> QSACTLQSETHPPLTWQKCSSGGTCTQQTGSVVIDANWRWTHATNSSTNCYDGNTWSSTLCPDNETCAKNCCLDGAAYASTYGVTTSGNSLSIDFVTQSAQKNVGARLYLMASDTTYQEFTLLGNEFSFDVDVSQLPCGLNGALYFVSMDADGGVSKYPTNTAGAKYGTGYCDSQCPRDLKFINGQANVEGWEPSSNNANTGIGGHGSCCSQMDIWEANSISEALTPHPCTTVGQEICEGDGCGGTYSDNRYGGTCDPDGCDWNPYRLGNTSFYGPGSSFTLDTTKK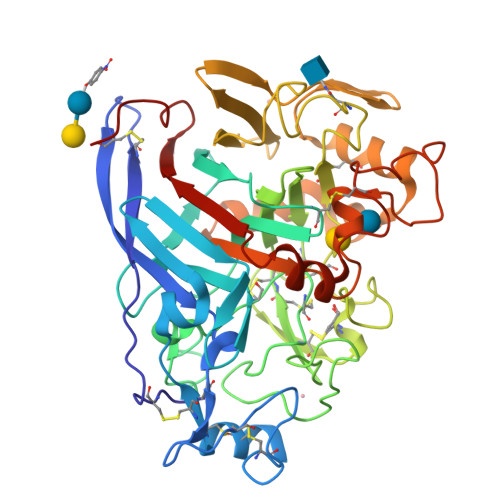LTVVTQFETSGAINRYYVQNGVTFQQPNAELGSYSGNELNDDYCTAEEAEFGGSSFSDKGGLTQFKKATSGGMVLVMSLWDDYYANMLWLDSTYPTNETSSTPGAVRGSCSTSSGVPAQVESQSPNAKVTFSNIKFGPIGSTGNPSG>[2x]ARDISIEDLLARKPKDLDDSAVAAFLKDKVVLVSGAGGTIGSELCKQCIKF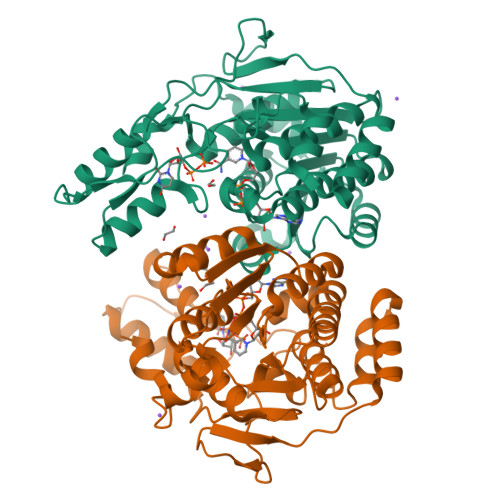GAKHLIMVDHSEYNLYKINDDLNLYKEKITPILLSILDKQSLDEVLKTYKPELILHAAAYKHVPLCEQNPHSAVINNILGTKILCDSAKENKVAKFVMISVDKAVRPTNIMGCTKRVCELYTLSMSDENFEVACVRFGNVLGSSGSVIPKFKAQIANNEPLTLTHPDIVRYFMLVAEAVQLVLQAGAIAKGGELFVLDMGKPVKIIDLAKKMLLLSNRNDLEIKITGLRKGEKLYEELLIDENDAKTQYESIFVAKNEKVDLDWLNKEIENLQICEDISEALLKIVPEFKHNKEGIAAGFNRIPAAALEHHHHHH>GSKISFPYLGKITHLKRLNHDTREIQIHLSRPFNYQSGQFAFLKIFQEGFESAPHPFSISGGHGQTLYFTVKTSGDHTKNIYDNLQAGSKVTLDRAYGHMIIEEGRENQVWIAGGIGITPFISYIREHPILDKQVHFYYSFRGDENAVYLDLLRNYAQKNPNFELHLIDSTKDGYLNFEQKEVPEHATVYMCGPISMMKALAKQIKKQNPKTELIYEGFKFK[3x]

NADPH oxidases (NOX) are transmembrane proteins, widely spread in eukaryotes and prokaryotes, that produce reactive oxygen species (ROS). The cytosolic dehydrogenase (DH) domain belongs to the Ferredoxin NADP +Reductase (FNR) family which has motifs to bind a flavin cofactor and a pyridine dinucleotide NAD(P)H. Thus, the NOX core catalytic domain contains the necessary machinery to move electrons from the electron donor – NADPH – through the flavin and heme cofactors to the ultimate electron acceptor, molecular oxygen, to make the ROS product. SpNOX purifies as a monomer and is constitutively active, so it represents the minimal functional core shared by all NOX family members. Here, we obtained X-ray structures of WT and F397W mutant of DH-only, and of a F397W mutant of full-length SpNOX.

To solve the SpNOXDH WT structure, we used the SpNOXDH F397W structure as a model, and achieved 2.5 Å resolution. As expected, SpNOXDH presents a typical fold of the FNR superfamily of reductase domain containing two sub-domains, the FAD-binding domain (FBD) and an NADPH-binding domain (NBD). Both WT and F397W SpNOXDH display 3 molecules per asymmetric unit and the two structures are identical. In the asymmetric unit of SpNOXDH WT, one of the three molecules contains no flavin. In the wild type, the isoalloxazine ring is sandwiched between FBD residues P234 and F235 on its si-face, and the NBD residue F397 on its re-face. Superposition of the different SpNOXDH WT molecules from the crystal asymmetric unit shows that the F397 aromatic ring imperfectly occupies the position in front of the re-face of the isoalloxazine ring, with orientation 40° with respect to the plane of the isoalloxazine ring, and distance at 5.3 Å. Phe in this position, however, leaves more space in this pocket and the sidechain has more degrees of freedom, making it feasible for the nicotinamide to displace it and transfer hydride to the isoalloxazine. The DH domain shows almost no contact with the ribitol and adenosine parts of the FAD. With the exception of possible polar contact of the first phosphate group with the backbone of the protein, the rest of the FAD molecule points out into the solvent, in the direction of the missing TM domain. From these observations, WT SpNOXDH could well behave as a flavin reductase, able to use different flavins as substrate through the sole recognition of the isoalloxazine ring. In contrast, the SpNOXDH retains constant affinity equal to that of lumiflavin (~10 μM) regardless of the flavin analog. These results suggest that the isolated DH domain binds to FAD primarily at the isoalloxazine ring of the cofactor, and the addition of ribitol (riboflavin), phosphate groups (FMN), and adenosine nucleotide (FAD) do not further interact significantly with the isolated DH domain.In the first step of the HP, GFAT synthesizes d-glucosamine-6-phosphate (GlcN6P) from l-glutamine (l-Gln) and Frc6P, releasing l-glutamate (l-Glu). GFAT contains two domains: the glutaminase domain responsible for releasing ammonia in the hydrolysis of l-Gln to l-Glu and the isomerase/transferase domain, which catalyzes both the isomerization of Frc6P to d-glucose-6-phosphate (Glc6P) as well as the transfer of ammonia to Glc6P to produce GlcN6P. The active sites of the two domains are linked by an ammonia channel, which forms when GFAT engages with both of its substrates, l-Gln and Frc6P. The main distinctive feature between prokaryotic and eukaryotic GFAT is the feedback inhibition by the HP product UDP-GlcNAc, which inhibits the glutaminase function.

To understand HP regulation at the molecular level, we determined the crystal structure of active full-length human GFAT-1. Tetragonal GFAT-1 crystals formed within a few days and diffracted to a resolution limit of 2.4 Å. GFAT-1 was crystallized in the presence of its substrate Frc6P and the product l-Glu. As the presence of the linear sugar suggests isomerization activity and the equilibrium constant for Frc6P-Glc6P-isomerization favors Glc6P formation, we decided to model the product Glc6P in our crystal structures. The product L-Glu is bound to the glutaminase active site in one monomer (monomer A), but is absent in the second monomer (monomer B). In the l-Glu-free state, Cys2 faces the substrate-binding pocket, while it points away from the active site in the presence of l-Glu. Due to the conformational shift of the glutaminase domains relative to their isomerase domains, the cleft between the two domains is more open in monomer A than in monomer B. This open conformation in monomer A allows conformational changes at the active sites with loop movements, which do not occur in the closed conformation in monomer B. l-Glu was found bound to the glutaminase domain of the open monomer A, while in monomer B no l-Glu was detected. Here, in the presence of the product l-Glu, the Q-loop (residues 95–102) covers the glutaminase site, as observed in the isolated glutaminase domain from E. coli. In addition, there is a conformational change of the neighboring R-loop (residues 31–36). l-Glu-induced shifts of the Q- and R-loops trigger side chain rotations of Tyr35 (R-loop) and Trp96 (Q-loop), destabilizing the C-loop. Although both active sites are occupied by ligands in monomer A, no ammonia channel connecting the glutaminase and the isomerase site is formed.

>[2x]MCGIFAYLNYHVPRTRREILETLIKGLQRLEYRGYDSAGVGFDGGNDKDWEANACKIQLIKKKGKVKALDEEVHKQQDMDLDIEFDVHLGIAHTRWATHGEPSPVNSHPQRSDKNNEFIVIHNGIITNYKDLKKFLESKGYDFESETDTETIAKLVKYMYDNRESQDTSFTTLVERVIQQLEGAFALVFKSVHFPGQAVGTRRGSPLLIGVRSEHKLSTDHIPILYRTGKDKKGSCNLSRVDSTTCLFPVEEKAVEYYFASDASAVIEHTNRVIFLEDDDVAAVVDGRLSIHRIKRTAGHHHHHHDHPGRAVQTLQMELQQIMKGNFSSFMQKEIFEQPESVVNTMRGRVNFDDYTVNLGGLKDHIKEIQRCRRLILIACGTSYHAGVATRQVLEELTELPVMVELASDFLDRNTPVFRDDVCFFLSQSGETADTLMGLRYCKERGALTVGITNTVGSSISRETDCGVHINAGPEIGVASTKAYTSQFVSLVMFALMMCDDRISMQERRKEIMLGLKRLPDLIKEVLSMDDEIQKLATELYHQKSVLIMGRGYHYATCLEGALKIKEITYMHSEGILAGELKHGPLALVDKLMPVIMIIMRDHTYAKCQNALQQVVARQGRPVVICDKEDTETIKNTKRTIKVPHSVDCLQGILSVIPLQLLAFHLAVLRGYDVDFPRNLAKSVTVE> INQVRPKLPLLKILHAAGAQGEMFTVKEVMHYLGQYIMVKQLYDQQEQHMVYCGGDLLGELLG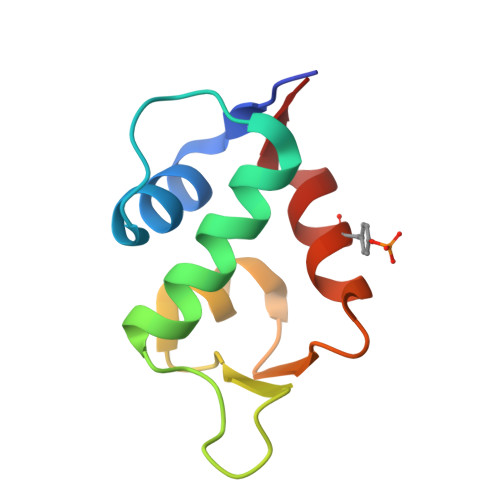RQSFSVKDPSPLYDMLRKNLVT>DQVDVKDCANNEIKKVMVDGC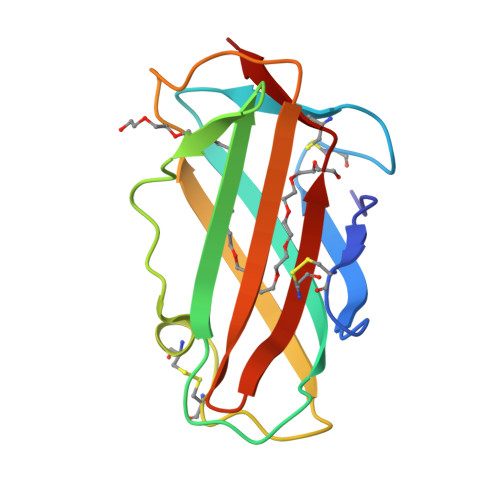HGSDPCIIHRGKPFTLEALFDANQNTKTAKIEIKASLDGLEIDVPGIDTNACHFMKCPLVKGQQYDAKYTWNVPKIAPKSENVVVTVKLVGDNGVLACAIATHAKIRD[2x]Protein CalO6 from the CAL gene cluster was originally proposed to catalyze one or both O-methylations (at positions C2 and/or C3) of this moiety. Homologues of CalO6 are dimeric SAM-dependent O-methyltransferases from bacteria and plants acting predominantly on hydroxyl groups of aromatic compounds involved in secondary metabolism. Methyltransferases of this family consist of three domains: the N-terminal helical domain is responsible for the dimerization via domain swapping, the central helical domain forms a lid over the active site, and the C-terminal Rossmann-fold domain bears a SAM binding motif and the catalytic residues, and forms a part of the substrate-binding pocket. Examples of such methyltransferases include caffeic acid O-methyltransferase from perennial ryegrass, human N-acetyl serotonin O-methyltransferase, as well as chalcone and isoflavone O-methyltransferases from alphalpha. It is proposed that the catalysis in these enzymes occurs through the activation of the hydroxyl group to be methylated through abstracting its hydrogen by a catalytic His residue in the enzyme active site (His252 in CalO6).

An example of challenging structure determination, CalO6, a dimeric Dnrk family O-methyltransferase, was crystallized in the absence of a cofactor or a substrate. The crystal structure of CalO6 was determined by a combination of molecular replacement by using diffraction data collected with native crystals with single anomalous dispersion (SAD) using an EMP derivative, as described in Materials and Methods. Locations of all mercury sites were consistent with covalent Cys modification. Crystals of CalO6 belong to space group R32, with one monomer in the asymmetric unit. The entirely helical N-terminal domain of CalO6 (residues 1 to 105) is involved in dimerization, and the C-terminal Rossman-fold domain (residues 162 to 356) containing the SAM-binding motif, is involved in substrate binding and the catalysis of the transfer of the methyl group from SAM onto a hydroxyl group of the substrate. A normally helical region between these two domains (residues 106 to 161; called a middle domain in some studies), which forms a part of the substrate-binding pocket in other methyltransferases, is disordered and not visible in the electron density map (as indicated by a dashed line in Fig. 4a). As a consequence, the substrate-binding pocket in CalO6 is much more open than in other O-methyltransferase structures. CalO6 appears to be the most extreme case, where the entire middle region is disordered or is in different positions relative to the rest of the protein in different CalO6 monomers in the crystal. The N-terminal domain is oriented at a different angle with respect to the catalytic domain from that seen in other methyltransferases bound to SAM, opening the active site even further.

> GSHMELTTTAARPGLRHRMQQLIYGFFTAQTLHVAVRLRIPDLLADGARDVGDLASATGADAPSLRRLLRALVFLEVLDEPAPGTFALTEQGEVLRADVTGSMRELVLLLSGPESWAAWGQLEHSVRTGEVAWEHVHGRSCFDHLMADPQRQAAFNAAMAEGSRAFVPTLLSAYDFGDLRTVVDVGGGSGALLAGVLAAHPHLRGTVFDTPDGVADAARTVAEQGVADRCGVETGDFFVSVPPGADAYVLKSVLHDWDDEQCVEVLRTVRRAVRPDSRVILVESLMPTTVTTAPSVAQVVMNDLNMMVCHGGRERTVAEFRELLRVAGFRLESVTPCPAPSVVGILEAAPAPATGPDGS> MPGLSCRFYQHKFPEVEDVVMVNVRSIAEMGAYVSLLEYNNIEGMILLSELSRRRIRSINKLIRIGRNECVVVIRVDKEKGYIDLSKRRVSPEEAIKCEDKFTKSKTVYSILRHVAEVLEYTKDEQLESLFQRTAWVFDDKYKRPGYGAYDAFKHAVSDPSILDSLDLNEDEREVLINNINRRLTPQAVKIRADIEVACYGYEGID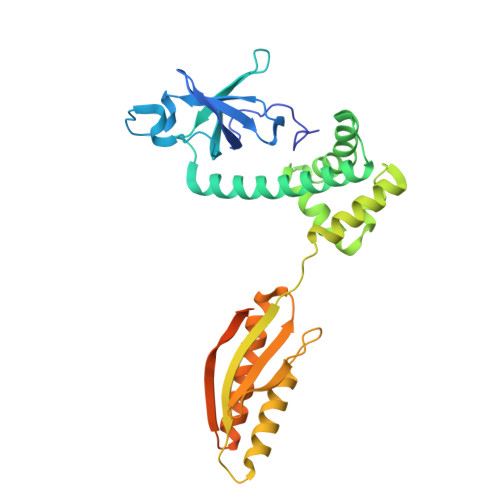AVKEALRAGLNCSTENMPIKINLIAPPRYVMTTTTLERTEGLSVLSQAMAVIKEKIEEKRGVFNVQMEPKVVTDTDETELARQMERLERENAEVDGDDDAEEMEAKAED> MSVKASGGSSLARPQLYQTVPVSAISQAEQQDRFLEGSELNELTAYFQSGALRLEIAETLTQNADLIVSRAANRIFTGGSPLSYLEKPVERQPALVGASSDSRNGSVTYAESNGSGGLFGGLRSVFSSTGPIPPGFRPINIARYGPSNMQKSLRDMSWFLRYTTYAIVAGDPNIIVVNTRGLKEVIENACSIDATIVAIQEMRAA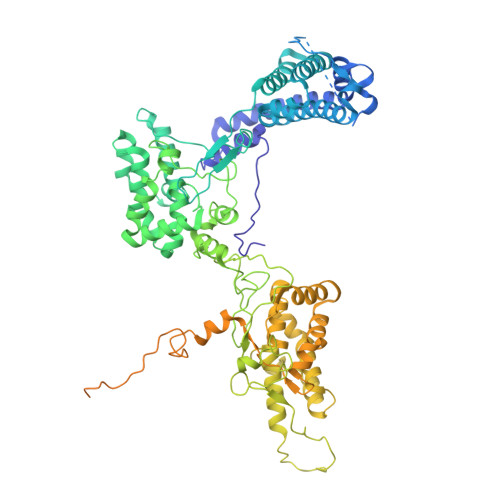SADYFRNNAQAKEIVLQYFDILLSEFKAPTPANKVRQGPSNDIQGLELPQSYFNAAAKRQKYAMKPGLSALEKNAVIKAAYRQIFERDITKAYSQSISYLESQVRNGDISMKEFVRRLAKSPLYRKQFFEPFINSRALELAFRHILGRGPSSREEVQKYFSIVSSGGLPALVDALVDSQEYADYFGEETVPYLRGLGVEAQECRNWGMQQDLFSYSAPFRKVPQFITTFAQYDRPLPDQHVYGSGNDPLEIQFGAIFPKETRNPSKRPAPFNKDTKRILIHRGPAVNNQVGNPSAVGEFPGSLGAKVFRLNGGLPGAKVGKNTGTSVKFGESSTQALIRAAYRQVFGRDLYEGQRLSVAEIQLENGDISVREFIKRLAKSELFLKLYWAPHYVCKAIEYMHRRLLGRPTYGRQEMNQYFDIASKQGFYAVVEAMIDSKEYSDAFGEDTVPYERYLTPGGLQMRSARVGSLREDIGQRVDKEVTPRFVELGQVSAIRTEPEIAYRSNQGVTRQRQQTKVFKLVSTYDKVAVKNAIRAAYRQVFERDLEPYIINSEFTALESKLSNNEINVKEFIEGLGTSELYMKEFYAPYPNTKVIEMGTKHFLGRAPLNQKEIQQYNQILASQGLKAFIGAMVNGMEYLQTFGEDTVPYRRFPTLPAANFPNTERLYNKLTKQDKELVVPSFTPVVKVGG>[2x]MDFTLSKQQQMVQKMYREFAENEVKPLAKKVDAEEYFPKETVEKMGKLGMMGIYFPTSVGGAGGDVLSYVMAVEELSKVCGTTGVIVSAHT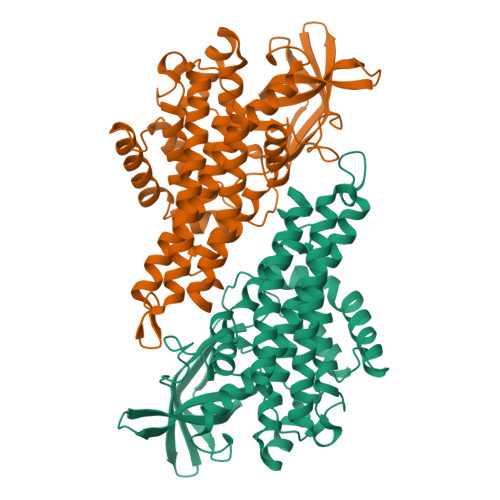SLCAAPIYENGTPEQKEKYLPKLCSGEWLGAFGLTEPGAGTDAQGQQTTAVEDGDYWVLNGSKIFITNAGYADVFIVIAVTDKVLDKKGRPTKLCSAFIVERTDPGFSVGKAEDKMGIRGSSTCELIFEDCRIPKDRMLGVRGKGFQLAMATLDGGRIGIASQALGIAEGALQETVAYVKERKQFGRSISAFQNTQFELAEMKARIEAAKYLVYAAALKKQEAMNGAKVRYSVEAAQAKLIAARTASDVTRRCLQLFGGYGYTRDYPIERMMRDAKITEIYEGTSEVQMMVISGALLK>GLGYGSWEIDPKDLTFLKELGTGQFGVVKYGKWRGQYDVAIKMIKEGSMSEDEFIEEAKVMMNLSHEKLVQLYGVCTKQRPIFIITEYMANGCLLNYLREMRHRFQTQQLLEMCKDVCEAMEYLESKQFLHRDLAARNCLVNDQGVVKVSDFGLSRYVLDDEYTSSVGSKFPVRWSPPEVLMYSKF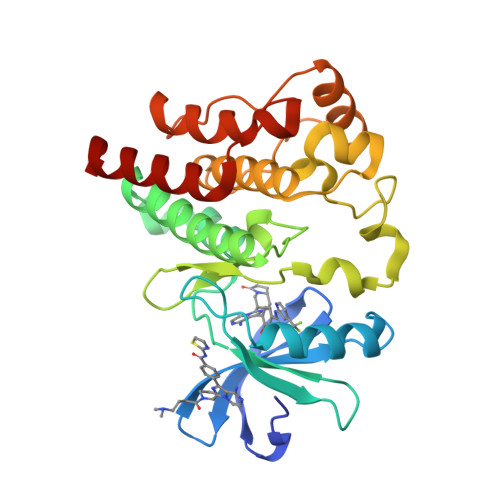SSKSDIWAFGVLMWEIYSLGKMPYERFTNSETAEHIAQGLRLYRPHLASEKVYTIMYSCWHEKADERPTFKILLSNILDVMDEES[2x]>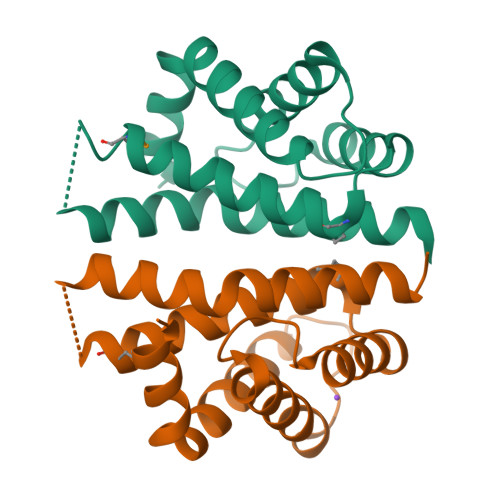[6x]MMSNQTVYQFIAENQNELLQLWTDTLKELSEQESYQLTDQVYENISKEYIDILLLSVKDENAAESQISELALRAVQIGLSMKFLATALAEFWKRLYTKMNDKRLPDQESTELIWQIDRFFSPINTEIFNQYSISWE>[2x]MTAVRRSTRIRTKSQVIEEDYDDEQNTSAQHVESDKITAKTQHEEEEEQDTGESEESSSEDDYEDQDDDDYVDTATAKRKSRKRKPKSASNTSSKRQKKKPTSAQKSAVSHAPAYHRSKKDQDQYLEIAKDFQPTELFDILSTSEDVSIEELLREWLETYSENRDKFLQEFINLLLNCCGSVARVEDHDVHSNESSNETIGEIQLLFQRQKLHEFYLLISKENKKRKNFKMGPLYQNFAEFMTKLLEVANDLQLLYVESDEDDTQIVTGNLVLDLLTWLSSFSVCKIRCFRYISTLTLYLFQDYLTQQAVNLEKNYLAKLSKQLSLEEKKKRPNNKTLEKLESTIAETQGSKVVIDSIID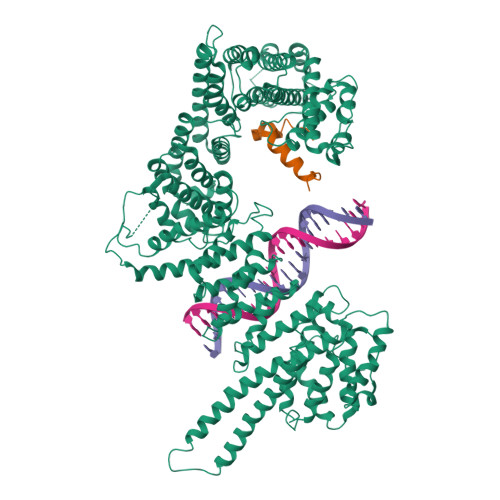NIVKLCFVHRYKDVSDLIRSESMLHLSIWIKNYPEYFLKVTFLKYFGWLLSDNSVSVRLQVTKILPHLIIQNHNSKSTDNSAIRQVFERFKTKILEVAIRDVNLDVRIHSIQVLTEASSLGYLDDSEILIISSLMFDEEFDPFKTSSFNKRSKFLSTVAKFLARVIKEKFDEFIKTHEDLPKEVDGLEVGPVVQVGIFIKILNDSLIYHLKDCAEVDSRTKIRMLTQAAEFLSPYISTHLKTICNLLISDTESNELIQKLQNSANNNSDDEDVDDEELDITPLFPIDRNSTILYLNVFHGLCAGANNPKIQTKDSVKEIVLPLFYDLLNAASIESADILCPLLESFITFSLDDWISIGYETELKKITDKTIKAFMDSTIGNSKVDMKYDIFAKFIHHIHHFEKKELQEKFLNQIATLKIHLKKFLQEKMDPNNSRDDYKDLTCSLYELYINKLTILGRDYPIEVDEELLQLFLNNFVSRIPIMFQDFDDSTAQEINFKMLVLLATWNLEKWREIIEKVRDYENSISKDLRSVWKPIAAIIGRLNTLVISLAATNETFENINSLFYLKWSACTSLMDIIVAIKIFELKLPADATTWRYSMSEQFPFYLHDNASKVLLKIFLYLESLFAKQVDVQLERVADEDANLNDLPETGFFENIETEFLLFTVKLKGLMKLNILDERFASRVALNKEKLGPLFKKIVDDTIMENPEPNKKNIQKAKSNQTQREKAPLQPNSERETDHANTENNDPDIPMTIDLEPIEESSQNNSELAPIEEHPTVVDAIDNSDEITQD;>TDAMTESQPKQTGTRRNSKLLNTKSIQIDEETENSESIASSNTYKEERSNNLLTPQPTNFTTKRLWSEITESMSYLPDPILKNFLSYESLKKRKIHNGRE[2x]>GGGGSMADPEVVVSSCSSHEEENRCNFNQQTSPSEELLLEDQMRRKLKFFFMNPCEKFWARGRKPWKLAIQILKIAMVTIQLVLFGLSNQMVVAFKEENTIAFKHLFLKGYMDRMDDTYAVYT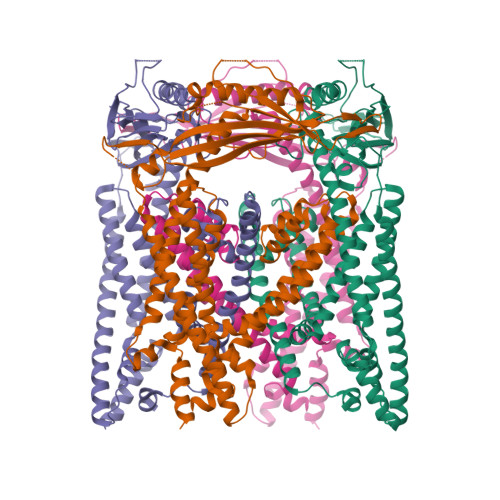QSDVYDQLIFAVNQYLQLYNVSVGNHAYENKGTKQSAMAICQHFYKRGNIYPGNDTFDIDPEIETECFFVEPDEPFHIGTPAENKLNLTLDFHRLLTVELQFKLKAINLQTVRHQELPDCYDFTLTITFDNKAHSGRIKISLDNDISIRECKDWHVSGSIQKNTHYMMIFDAFVILTCLVSLILCIRSVIRGLQLQQEFVNFFLLHYKKEVSVSDQMEFVNGWYIMIIISDILTIIGSILKMEIQAKSLTSYDVCSILLGTSTMLVWLGVIRYLGFFAKYNLLILTLQAALPNVIRFCCCAAMIYLGYCFCGWIVLGPYHDKFRSLNMVSECLFSLINGDDMFATFAKMQQKSYLVWLFSRIYLYSFISLFIYMILSLFIALITDTYETIKQYQQDGFPETELRTFISECKDLPNSGKYRLEDDPPVSLFCCCKK[4x]>MDKTVKLWNRNGQLLQTLTGHSSSVTGVAFSPDGQTIASASDDKTVKLWNRNGQLLQTLTGHSSSVTGVAFSPDGQTIASASDDKTVKLWNRNGQLLQTLTGHSSSVTGVAFSPDGQTIASASDD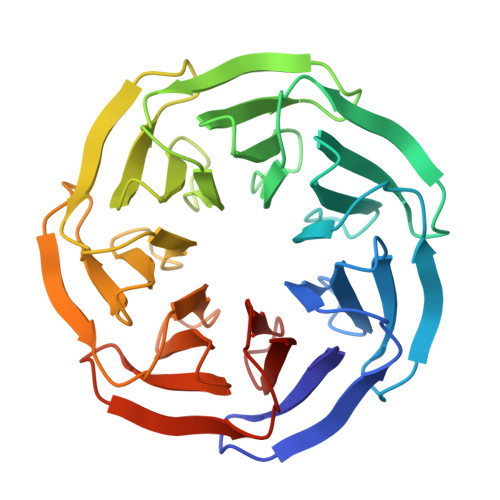KTVKLWNRNGQLLQTLTGHSSSVTGVAFSPDGQTIASASDDKTVKLWNRNGQLLQTLTGHSSSVTGVAFSPDGQTIASASDDKTVKLWNRNGQLLQTLTGHSSSVTGVAFSPDGQTIASASDDKTVKLWNRNGQLLQTLTGHSSSVTGVAFSPDGQTIASASD[4x]>MEEPKYTIDLRTNNGWWARLKSWFVGGRLVTPNQGSQTGPVSAHGYLGDSSINDERILQISTVWRCVSLISTLTACLPLDVFETDQNDNRKKVDLSNPLARLLRYSPNQYMTAQEFREAMTMQLCFYGNAYALVDRNSAGDVISLLPLQSANMDVKLVGKKVVYRYQRDSEYADFSQKEIFHLKGFGFTGLVGLSPIAFACKSAGVAVAMEDQQRDFFANGAKSPQILSTGEKVLTEQQRSQVEENFKEIAGGPVKKRLWILEAGFSTS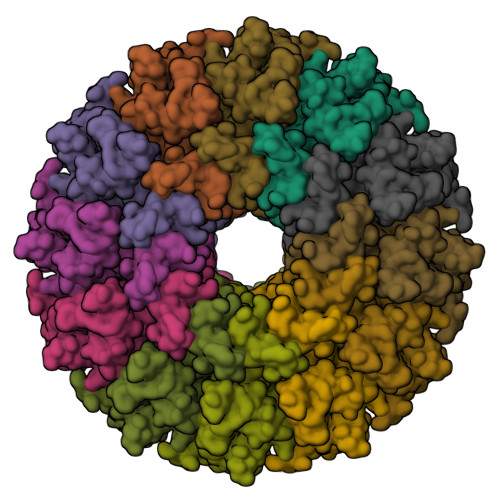AIGVTPQDAEMMASRKFQVSELARFFGVPPHLVGDVEKSTSWGSGIEQQNLGFLQYTLQPYISRWENSIQRWLIPSKDVGRLHAEHNLDGLLRGDSASRAAFMKAMGESGLRTINEMRRTDNMPPLPGGDVAMRQAQYVPITDLGTNKEPRNNGA[12x]> GPGYNEPQDKKTMMMNEEDDGNGMDELLAVLGYKVRSSEMADVAQKLEQLEVMMSNVQEDDLS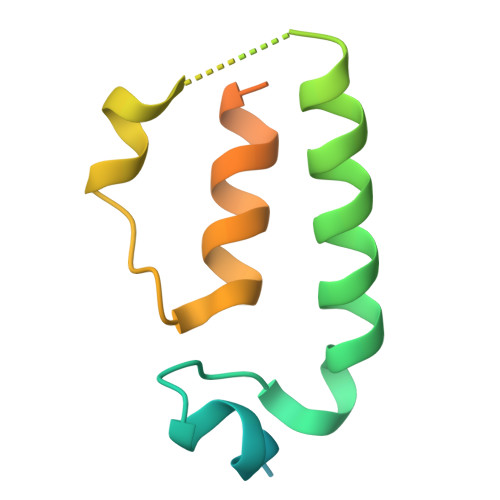QLATETVHYNPAELYTWLDSMLTDLNPPSSNAEYDLKAIPGDAILNQ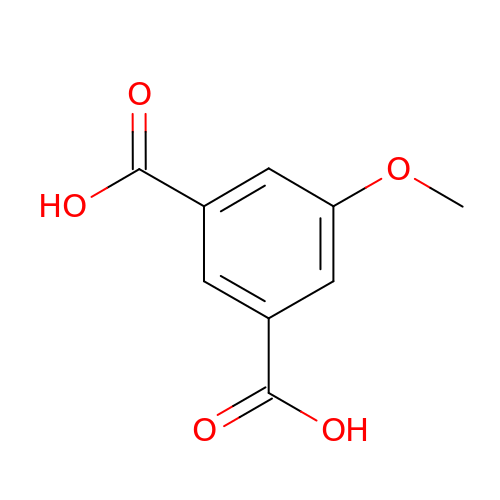5-methoxybenzene-1,3-dicarboxylic acid | C9 H8 O5 | POSMIIJADZKUPL-UHFFFAOYSA-N>[4x]GAMGMGLAGGSLPSLAPDLVRDLIATAADISLLVSQEGVVREVMANPHHPSFGQLSEWEGRPLEEVLTAESVAKFRLRSEGLEPGRGSVAVELNHIDPRSFEFPIRYILHRLPADRSILMLGRDLRPIAEVQQQLVAAQLAMERDYETQREMETRYRVVLDVSRDPMVLVSMSTGRIVDLNSAAGLLLGGV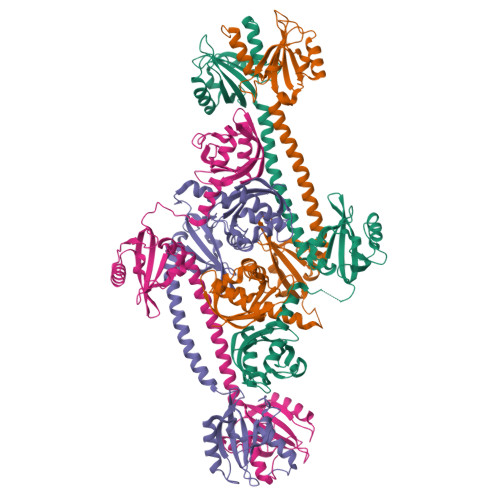RQDLLGAAIAQEFEGRRRGEFMETMTNLAATESAAPVEVLARRSQKRLLVVPRVFRAAGERLLLCQIDPADATQPVGDELSENLARLYHEGVDGIVFSDADGTIRGANEAFLNMTDSSSLAAIRGRSIADFLARGSVDLRVLIDSVRRTGQLRLYATRLTTDFAGQIAAEISATWLDDRERPLLVLVVRDTSR4-[(propan-2-yl)oxy]-N-{(4M)-4-[1-(2,2,2-trifluoroethyl)-1H-pyrazol-4-yl]quinolin-8-yl}benzamide | C24 H21 F3 N4 O2 | 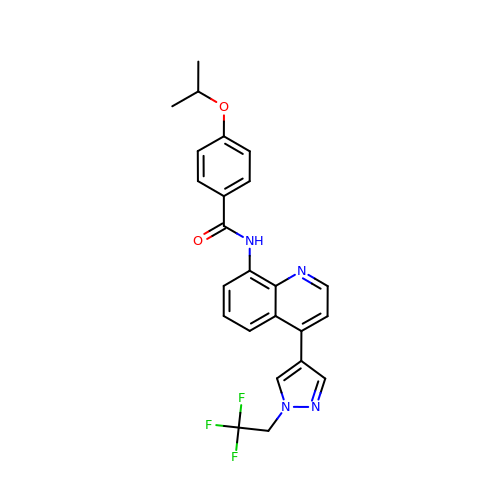BYJFUIUIQRINQL-UHFFFAOYSA-N> MNNNKRSKLSTVPSSRPIRVGFVGLTSGKSWVAKTHFLAIQQLSSQFQIVALYNPTLKSSLQTIEQLQLKHATGFDSLESFAQYKDIDMIVVSVKVPEHYEVVKNILEHSSQNLNLRYLYVEWALAASVQQAEELYSISQQRANLQTIICLQGRKSPYIVRAKELISEGCIGDINSIEISGNGG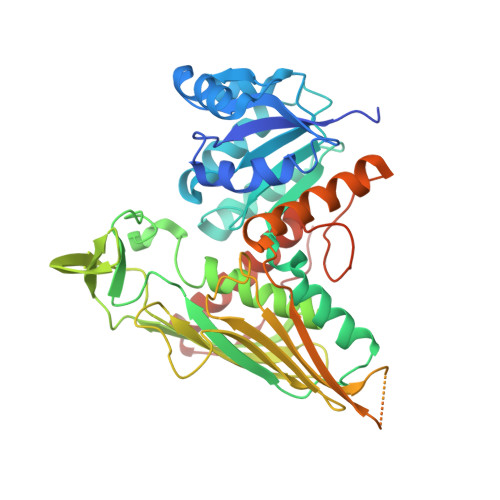WYGYERPMRSPEYLYDIESGVNLISNSFGHTIDVLQYITGSYFQKINAMISNNIPTQFLLDENGKRTKETISKTCPDHLLFQGILENGKVPVSCSFKGGTPVKKLTKNLVIDIHGTKGDLKIEGDAGFVEISNLVLYFYGIKNGNGSSNGTDNNGAAAIKDKEKVTKSPSPSTGTSEEEQTMEVFHLRNYNSVVGNILRIYESIADYHFLGKPESKSSRGPDDLFASTKFDKQGFRFEGFPTFKDAIILHRLIDAVFRSDKEEKTLDVSKIMILEHHHHHH> MELIEVQEGKAKILIPKAESIYDSPVFYNPRMALNRDIVVVLLNILNPKIVLDALSATGIRGIRFALETPAEEVWLNDISEDAYELMKRNVMLNFDGELRESKGRAILKGEKTIVINHDDANRL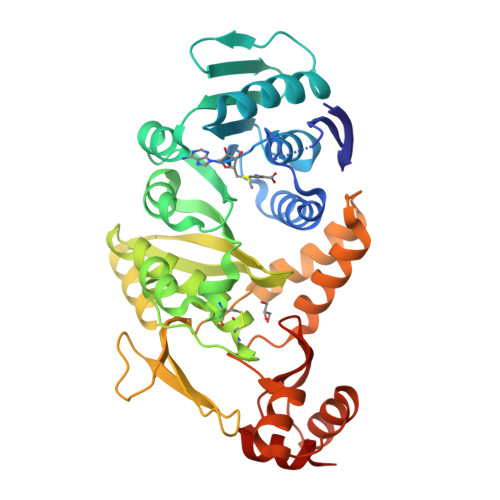MAERHRYFHFIDLDPFGSPMEFLDTALRSAKRRGILGVTATDGAPLCGAHPRACLRKYLAVPLRGELCHEVGTRILVGVIARYAAKYDLGIDVILAYYKDHYFRAFVKLKDGARKGDETLEKLGYIYFDDKTGKFELEQGFLPTRPNAYGPVWLGPLKDEKIVSKMVKEAESLSLARKKQALKLLKMIDQELDIPLFYDTHAIGRRLKIETKKVEEIISALREQGYEATRTHFSPTGIKTSAPYEVFIETIKRI> MASEIHMTGPMCLIENTNGRLMANPEALKILSAITQPMVVVAIVGLYRTGKSYLMNKLAGKKKGFSLGSTVQSHTKGIWMWCVPHPKKPGHILVLLDTEGLGDVEKGDNQNDSWIFALAVLLSSTFVYNSIGTINQQAMDQLYYVTELTHRIRSKSSPDENENEVEDSADFVSFFPDFVWTLRDFSLDLEADGQPLTPDEYLTYSLKLKKGTSQKDETFNLPRLCIRKFFPKKKCFVFDRPVHRRKLAQLEKLQDEELDPEFVQQVADFCSYIFSNSKTKTLSGGIQVNGPRLESLVLTYVNAISSGDLPCMENAVLALAQIENSAAVQKAIAHYEQQMGQKVQLPTESLQELLDLHRDSEREAIEVFIRSSFKDVDHLFQKELAAQLEKKRDDFCKQNQEASSDRCSGLLQVIFSPLEEEVKAGIYSKPGGYRLFVQKLQDLKKKYYEEPRKGIQAEEIL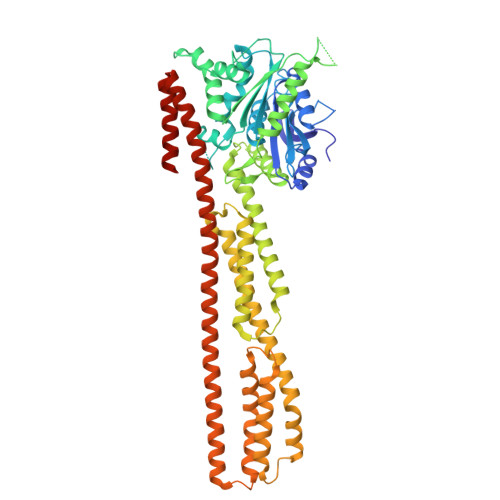QTYLKSKESMTDAILQTDQTLTEKEKEIEVERVKAESAQASAKMLHEMQRKNEQMMEQKERSYQEHLKQLTEKMENDRVQLLKEQERTLALKLQEQEQLLKEGFQKESRIMKNEIQDLQTKMRRRKACTIS> GHMSGEAPLTATVDGIIQPMLKAYRIPGMAVAVLKDGKAHYFNYGVANRESGQRVSEQTLFEIGSVSKTLTATLGAYAAVKGGFELDDKVSQHAPWLKGSAFDGVTMAELATYSAGGLPLQFPDEVDSNDKMQTY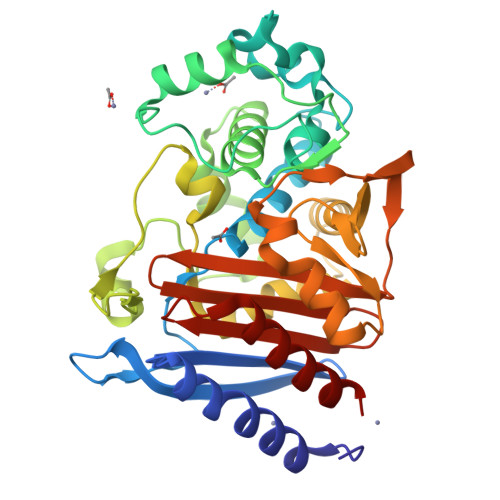YRSWSPVYPAGTHRQFSNPSIGLFGHLAANSLGQPFEQLMSQTLLPKLGLHHTYIQVPESAMANYAYGYSKEDKPIRATPGVLAAEAYGIKTGSADLLKFVEANMGYQGDAALKSAIALTHTGFHSVGEMTQGLGWESYDYPVTEQVLLAGNSPAVSFQANPVTRFAVPKAMGEQRLYNKTGSTGGFGAYVAFVPARGIAIVMLANRNYPIEARVKAAHAILSQLAE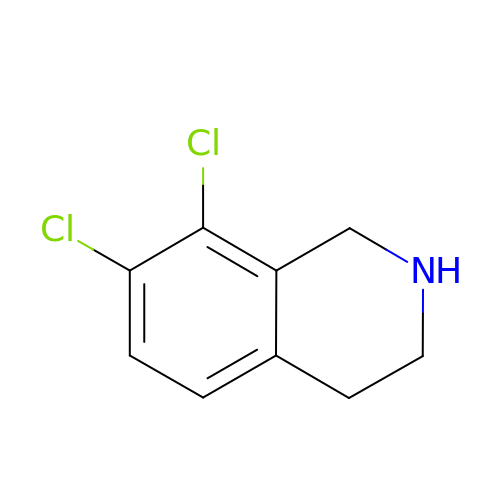7,8-DICHLORO-1,2,3,4-TETRAHYDROISOQUINOLINE | C9 H9 Cl2 N | WFPUBEDBBOGGIQ-UHFFFAOYSA-N> KPEPTDEEWELIKTVTEAHVATNAQGSHWKQKRKFLPEDIGQAPIVNAPEGGKVDLEAFSHFTKIITPAITRVVDFAKKLPMFCELPCEDQIILLKGCCMEIMSLRAAVRYDPESETLTLNGEMAVTRGQLKNGGLGVVSDAIFDLGMSLSSFNLDDTEVALLQAVLLMSSDRPGLACVERIEKYQDSFLLAFEHYINYRKHHVTHFWPKLLMKVTDLRMIGACHASWFLHMKVECPTELFPPLFLEVFE;> ENALLRYLLDK

The thyroid hormone receptors (THRs) are nuclear hormone receptors regulated by endogenous thyroid hormones, including the inactive prohormone thyroxine (T4) and the bioactive hormone 3,3′,5-triiodothyronine (T3), which are critical for development regulation and metabolic homeostasis. As ligand-regulated nuclear receptors, THRs have a structurally conserved LBD that allows the binding of distinct ligands (Burris et al., 2013). Following the ligand binding, the function of THRs is mediated through the selective recruitment or release of specific coregulators, like the family of steroid receptor coactivators (SRCs) (Li et al., 2003, Jin and Li, 2010, Savkur and Burris, 2004), as a heterodimeric complex with retinoid X receptor (RXR) (Putcha et al., 2012, Kojetin et al., 2015, Mangelsdorf and Evans, 1995). Although the defects in any of the processes in thyroid hormone transport and synthesis can all contribute to RTH, in most cases the disorder involves defective thyroid hormone receptors, resulting in reduced T3 binding and disruptive thyroid hormone signaling.

As expected, the native ligand T3 abolished or substantially diminished the transcriptional activity of four THRβ mutants associated with thyroid hormone resistance, V264D, H435L, R438H, and R438W, respectively (Wakasaki et al., 2016, Nomura et al., 1996, Sabet and Pallotta, 2011, Narumi et al., 2010). Surprisingly, the treatment of roxadustat either enhanced or retained the transcriptional activity of these THRβ mutants, all leading to higher induced transcriptional activity than those of T3. In contrast, the binding of roxadustat resulted in higher Tm values for four TRβ mutants than that of T3. Although all four mutant residues are located in the THRβ LBD, H435 is the only one that directly contacts ligands T3 or roxadustat, whereas the rest of the mutant residues are located outside the ligand-binding pocket, not in the range to form intimate contacts with the ligands, which makes us wonder how these mutants influence the ligand binding. To unravel the molecular basis for the RTH of the THRβ mutants and further their beneficial susceptibility to roxadustat, we performed structural studies on the THRβ mutants complexed with roxadustat. The structural analysis further revealed an apparent conformational change of residue H435 on helix 10 of THRβ for all four mutants, resulting in the loss of a critical hydrogen bond between THRβ and a critical hydroxy group of T3, which is also conserved for the other THR ligands identified so far, explaining the severely reduced THRβ activity by T3. Specifically, in addition to the direct mutation of H435 to the hydrophobic leucine of THRβ H435L, the allosteric conformational changes of THRβ H435 were coupled with several intermediate structural changes, predominantly in helix 10, which were initiated by mutants R438H, R438W, or V264D, consequently leading to impaired T3 binding.>ATTDAECLSKPAFDGTLSNVWKEGDSRYANFENCIYELSGI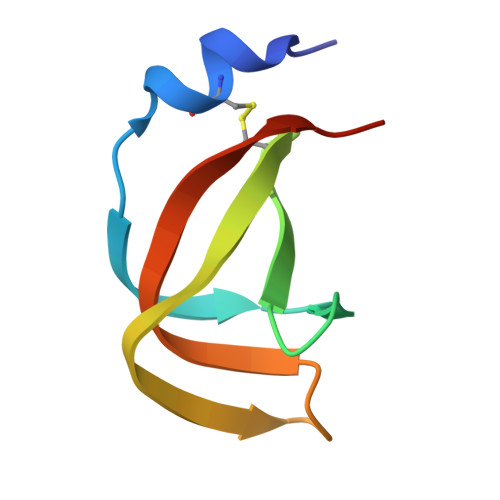GIGYDNDTSWNGHWTPVRAADGSG[2x]> RTLLSLGLLVADFGAMVNNPHLSDVQFQTDSGEVLYAHKFVLYARCPLL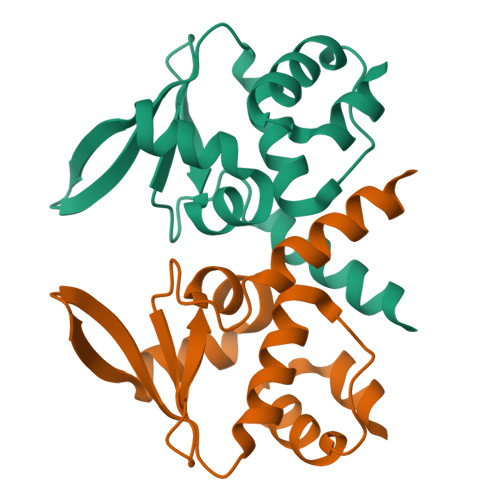IQYVNNEGFSAVEDGVLTQRVLLGDVSTEAARTFLHYLYTADTGLPPGLSSELSSLAHRFGVSELVHLCE>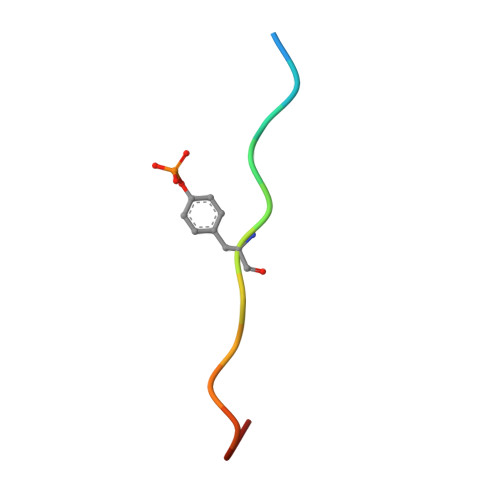 XEEENIYSVPHDST> GNYENINSNPYEAPDLSADGYALGSAMNNLAGCVVSPDVNTAQFTDCLLGGPLGGYFADSNAGFTETISNFNPKDDWSRVFLKSDKIIPTLYSNLTQVKLVSQNTNDPVPYAIAQVIKVAAMHRVTDAFGPIPYSQIGANGEIATPYDSQEVTYNTFFDELNAAIATLNENSNEQLVPTADYIYKGDVKKWIRFANSLKLRLAIRIAYANPVKAQQMAEEAVNPANGGVIESNADNATWNYFETSQNPIYVATRYNQVQTSDHGGVPCLTGGDTHAAADIICYMNGYKDNRREKFFTKSEWAGQDYVGMRRGIVIPELKTTGHKYSGVNIAPTSPLYWMNAAEVAFLRAEGQAVFN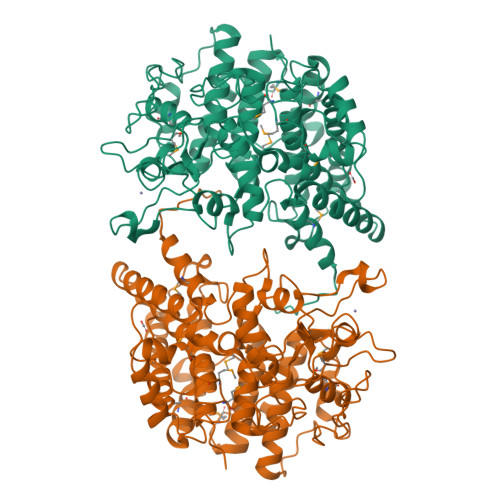FSMGGTAESFYNQGIRLSFEQWGADGVEDYLKDDVNKPTAYTDPAGTNTYQNALSNITIKWNDSADKEEKQERIIVQKWIANWQLGNEAWADFRRTGYPKLIPVKENKSGGVVDSEKGARRMPYPLDEFVSNKANVEYAIANYLHGADNMATDVWWASKK N-[(S)-({[(benzyloxy)carbonyl]amino}methyl)(hydroxy)phosphoryl]-L-phenylalanyl-L-leucine | C24 H32 N3 O7 P | 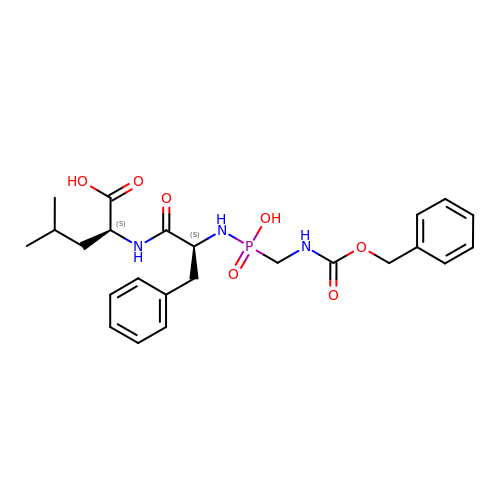XQFJAKNVSJXHDS-SFTDATJTSA-N>GPKFPRVKNWELGSITYDTLCAQSQQDGPCTPRRCLGSLVLPRKLQTRPSPGPPPAEQLLSQARDFINQYYSSIKRSGSQAHEERLQEVEAEVASTGTYHLRESELVFGAKQAWRNAPRCVGRIQWGKLQVFDARDCSSAQEMFTYICNHIKYATNRGNLRSAITVFPQRAPGRGDFRIWNSQLVRYAGYRQQDGSVRGDPANVEITELCIQHGWTPGNGRFDVLPLLLQAPDEAPELFVLPPELVLEVPLEHPTLEWFAALGLRWYALPAVSNMLLEIGGLEFSAAPFSGWYMSTEIGTRDLCDPHRYNILEDVAVCMDLDTRTTSSLWKDKA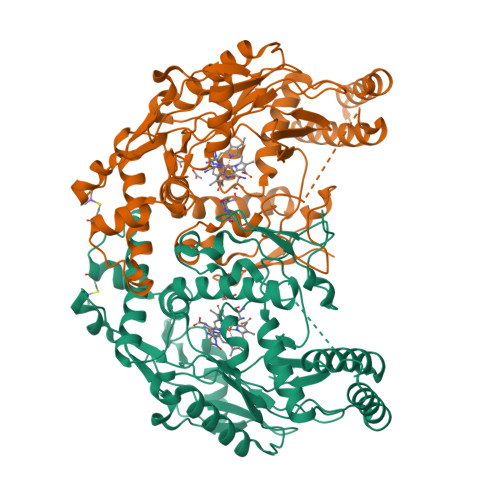AVEINLAVLHSFQLAKVTIVDHHAATVSFMKHLDNEQKARGGCPADWAWIVPPISGSLTPVFHQEMVNYILSPAFRYQPDPW[2x]> MLRESFAISGDSLISLASTGKRVPIKDLLGEKDFEIWAINEQTMKLESAKVSRVFCTGKKLVYTLKTRLGRTIKATANARFLTIDGWKRLDELSLKEHIALPRKLESSSLQLAPEIEKLPQSDIYWDPIVSITETGVEEVFDLTVPGLRNFVANDIIVHASIEQDKLGG

Inteins are protein elements that remove themselves from their precursor proteins in an autocatalytic pathway called protein splicing. In the first step of the canonical class 1 inteins, the scissile peptide bond upstream of the intein rearranges in an N–S (or N–O) acyl shift involving the cysteine (or serine) side chain as the first amino acid of the intein (residue 1) and the upstream flanking amino acid of the N-extein (residue (–1)). The M86 mutant of the Ssp DnaB intein (here referred to as WT intein) was selected by sequential directed evolution for its more general activity and is one of the few known intein mutants with improved extein promiscuity.

Strikingly, the functional complementation of the catalytic His73 through a large (–1) side chain also extended to a single H73A mutant of the M86 intein. Here, splicing activity was restored, whereas the same intein with the native Gly(–1) was completely inactive. Again, this hypothesis was confirmed by the crystal structure of the G(–1)F/H73A mutant, which revealed that significant changes are indeed restricted to the N-terminal splice junction. The effects are even more pronounced in the M86(G(–1)F/H73A) mutant. Here, the dihedral angle φ of the Ala1 residue is twisted to –76°, which represents a marked change of up to 91° relative to the other M86 structures. The resulting twist rotates the carbonyl of the scissile peptide bond toward the space liberated by the missing His73 side chain. The new space has also accommodated a water molecule (water 5), which is not present in the other two structures. This water molecule seems to stabilize the twisted conformation by coordinating the carbonyl oxygens of Phe(–1) and of the block G His153. The overall distortion of the plane with the scissile peptide bond, described by the angle ω, increases from the M86 intein (ω = 179°) to the G(–1)F mutant (ω = –173°) and the G(–1)F/H73A double mutant (ω = –159°). In particular the latter structure, with 21° off from the optimal trans-conformation, suggests that the mutations have a significant effect on the stability of the peptide bond.>MDIAIHHPWIRRPFFPFHSPSRLFDQFFGEHLLESDLFPTSTSLSPFYLRPPSFLRAPSWFDTGLSEMRLEKDRFSVNLDVKHFSPEELKVKVLGDVIEVHGKHEERQDEHGFISREFHRKYRIPADVDPLTITSSL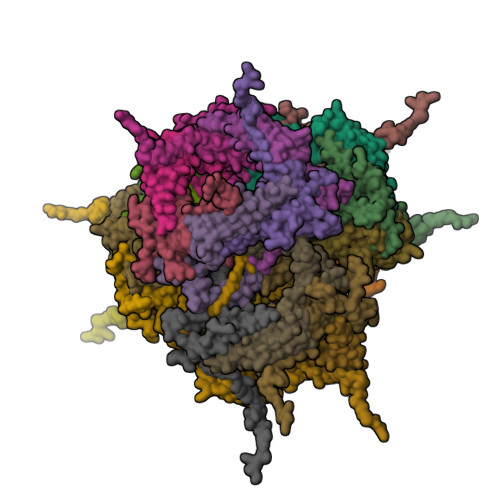SSDGVLTVNGPRKQVSGPERTIPITREEKPAVTAAPKK[24x]> MERYENLFAQLNDRREGAFVPFVTLGDPGIEQSLKIIDTLIDAGADALELGVPFSDPLADGPTIQNANLRAFAAGVTPAQCFEMLALIREKHPTIPIGLLMYANLVFNNGIDAFYARCEQVGVDSVLVADVPVEESAPFR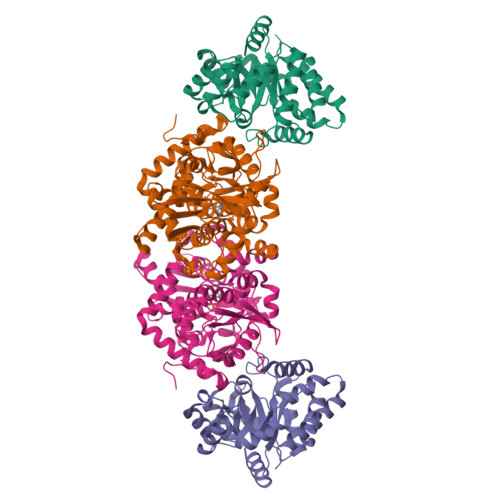QAALRHNIAPIFICPPNADDDLLRQVASYGRGYTYLLSRSGVTGAENRGALPLHHLIEKLKEYHAAPALQGFGISSPEQVSAAVRAGAAGAISGSAIVKIIEKNLASPKQMLAELRSFVSAMKAASRA;> TTLLNPYFGEFGGMYVPQILMPALNQLEEAFVSAQKDPEFQAQFADLLKNYAGRPTALTKCQNITAGTRTTLYLKREDLLHGGAHKTNQVLGQALLAKRMGKSEIIAETGAGQHGVASALASALLGLKCRIYMGAKDVERQSPNVFRMRLMGAEVIPVHSGSATLKDACNEALRDWPGSYETAHYMLGTAAGPHPYPTIVREFQRMIGEETKAQILDKEGRLPDAVIACVGGGSNAIGMFADFINDTSVGLIGVEPGGHGIETGEHGAPLKHGRVGIYFGMKAPMMQTADGQIEESYSISAGLDFPSVGPQHAYLNSIGRADYVSITDDEALEAFKTLCRHEGIIPALESSHALAHALKMMREQPEKEQLLVVNLSGRGDKDIFTVHDILKARGEI5-chloro-N-{[(4R)-2,5-dioxo-4-(1,3-thiazol-2-yl)imidazolidin-4-yl]methyl}-1-benzofuran-2-carboxamide | C16 H11 Cl N4 O4 S | 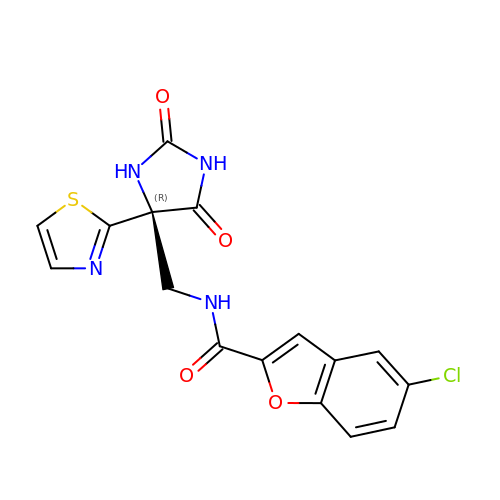LBVBVIKJOWWVJX-MRXNPFEDSA-N> GPKKISNCSKIHLSTKLLAVDFPAHFVKSISCQICEHILADPVETSCKHLFCRICILRCLKVMGSYCPSCRYPCFPTDLESPVKSFLNILNSLMVKCPAQDCNEEVSLEKYNHHVSSHKESKETLVHINKGGRPRQHLLSLTRRAQKHRLRELKIQVKEFADKEEGGDVKAVCLTLFLLALRARNEHRQADELEAIMQGRGSGLQPAVCLAIRVNTFLSCSQYHKMYRTVKAITGRQIFQPLHALRNAEKVLLPGYHPFEWQPPLKNVSSRTDVGIIDGLSGLASSVDEYPVDTIAKRFRYDSALVSALMDMEEDILEGMRSQDLDDYLNGPFTVVVKESCDGMGDVSEKHGSGPAVPEKAVRFSFTVMRITIEHGSQNVKVFEEPKPNSVLCCKPLCLMLADESDHETLTAILSPLIAEREAMKSSELTLEMGGIPRTFKFIFRGTGYDEKLVREVEGLEASGSVYICTLCDTTRLEASQNLVFHSITRSHAENLQRYEVWRSNPYHESVEELRDRVKGVSAKPFIETVPSIDALHCDIGNAAEFYKIFQLEIGEVYKHPNASKEERKRWQATLDKHLRKRMNLKPIMMMNGNFARKLMTQETVDAVCELIPSEERHEALRELMDLYLKMKPVWRSSCPAKECPESLCQYSFNSQRFAE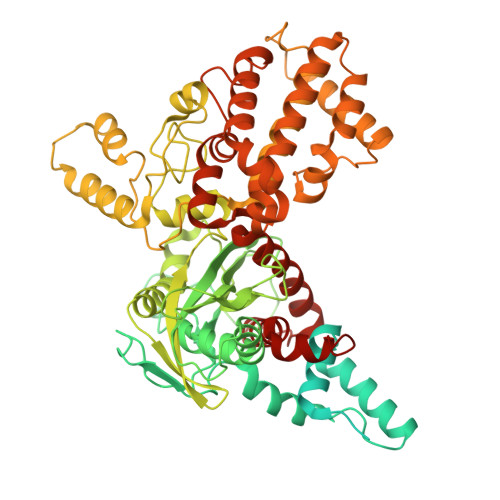LLSTKFKYRYEGKITNYFHKTLAHVPEIIERDGSIGAWASEGNESGNKLFRRFRKMNARQSKCYEMEDVLKHHWLYTSKYLQKFMNAHNA2-DEOXY-ADENOSINE -5'-THIO-MONOPHOSPHATE 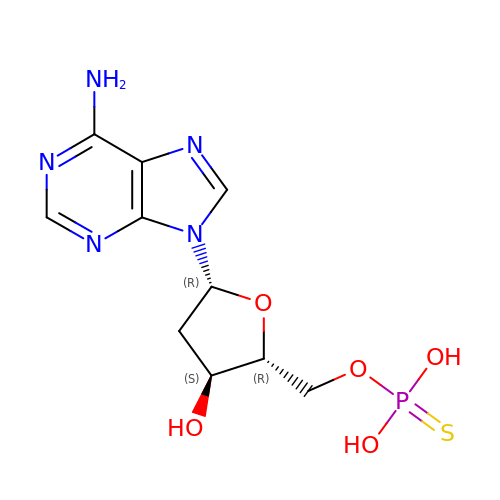| C10 H14 N5 O5 P S | ULJYSQHUKIZEGB-RRKCRQDMSA-N> TEMSVRKIAAHMKSNPNAKVIFMVGAGISTSCGIPDFRSPGTGLYHNLARLKLPYPEAVFDVDFFQSDPLPFYTLAKELYPGNFRPSKFHYLLKLFQDKDVLKRVYTQNIDTLERQAGVKDDLIIEAHGSFAHCHCIGCGKVYPPQVFKSKLAEHPIKDFVKCDVCGELVKPAIVFFGEDLPDSFSETWLNDSEWLREKITTSGKHPQQPLVIVVGTSLAVYPFASLPEEIPRKVKRVLCNLETVGDFKANKRPTDLIVHQYSDEFAEQLVEELGWQEDFEKILTAQ

Lysine benzoylation (Kbz) is a recently discovered post-translational modification associated with active transcription. Here, we systematically characterize writer, eraser, and reader proteins of histone Kbz in S. cerevisiae using proteomic, biochemical, and structural approaches. The Spt-Ada-Gcn5 acetyltransferase (SAGA) complex and NAD+-dependent histone deacetylase Hst2 could function as the writer and eraser of histone Kbz, respectively. In addition, we demonstrate that a subset of YEATS domains and bromodomains serve as Kbz readers, and structural analyses reveal how YEATS and bromodomains recognize Kbz marks.

We also tried to crystallize the ternary complex composed of Hst2, benzoylated substrate, and cofactor NAD+, but the solved complex structure at 1.8 Å only showed the density of 2’-O-benzoyl-ADP-ribose, the cofactor product. We presumed that the ternary complex initially formed and reacted, producing 2’-O-benzoyl-ADP-ribose that remained bound while the debenzoylated substrate and nicotinamide dissociated. The appearance of 2’-O-benzoyl-ADP-ribose also suggests that the debenzoylation process utilizes a similar catalytic mechanism as deacetylation catalyzed by NAD+-dependent HDACs. In both structures, Hst28-294 exhibits an elongated structure containing a large Rossmann-fold domain and a small zinc-containing domain. The small domain consists of four α-helices (α3-5, α9) and three β-strands (β4-6). Both the H3 peptide and the cofactor product bind to the cleft between two domains. The superimposition of two structures by the large domains shows a 17° rotation of the small domain and the rearrangement of the α2–α3 loop involved in contacting the 2′-O-benzoyl-ADP-ribose. Such rigid body rotation might be facilitated by four glycine residues serving as hinges located at junctions between the large domain and the small domain.>[2x]MEPEAPRRRHTHQRGYLLTRNPHLNKDLAFTLEERQQLNIHGLLPPSFNSQEIQVLRVVKNFEHLNSDFDRYLLLMDLQDRNEKLFYRVLTSDIEKFMPIVYTPTVGLACQ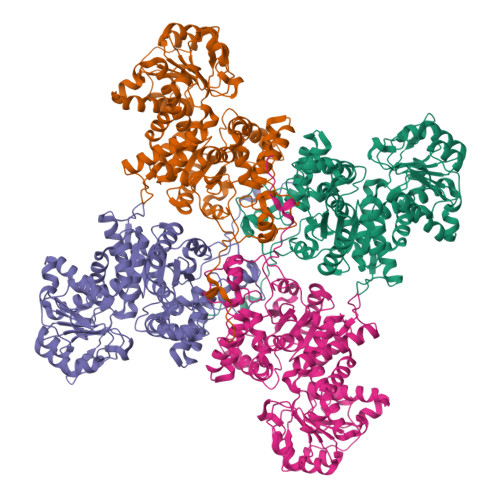QYSLVFRKPRGLFITIHDRGHIASVLNAWPEDVIKAIVVTDGERILGLGDLGCNGMGIPVGKLALYTACGGMNPQECLPVILDVGTENEELLKDPLYIGLRQRRVRGSEYDDFLDEFMEAVSSKYGMNCLIQFEDFANVNAFRLLNKYRNQYCTFNDDIQGTASVAVAGLLAALRITKNKLSDQTILFQGAGEAALGIAHLIVMALEKEGLPKEKAIKKIWLVDSKGLIVKGRASLTQEKEKFAHEHEEMKNLEAIVQEIKPTALIGVAAIGGAFSEQILKDMAAFNERPIIFALSNPTSKAECSAEQCYKITKGRAIFASGSPFDPVTLPNGQTLYPGQGNNSYVFPGVALGVVACGLRQITDNIFLTTAEVIAQQVSDKHLEEGRLYPPLNTIRDVSLKIAEKIVKDAYQEKTATVYPEPQNKEAFVRSQMYSTDYDQILPDCYSWPEEVQKIQTKVDQLEHHHHHH> QKPKYQVRWKIIESYEGNSYTFIDPTQLPYNEKWEFPRNNLQFGKTLGAGAFGKVVEATAFGLGKEDAVLKVAVKMLKSTAHADEKEALMSELKIMSHLGQHENIVNLLGACTHGGPVLVITEYCCYGDLLNFLRRKAEAMLGPSLSPGQDPEGLDKEDGRPLELRDLLHFSSQVAQGMAFLASKNCIHRDVAARNVLLTNGHVAKIGDFGLARDIMNDSNYIVKGNARL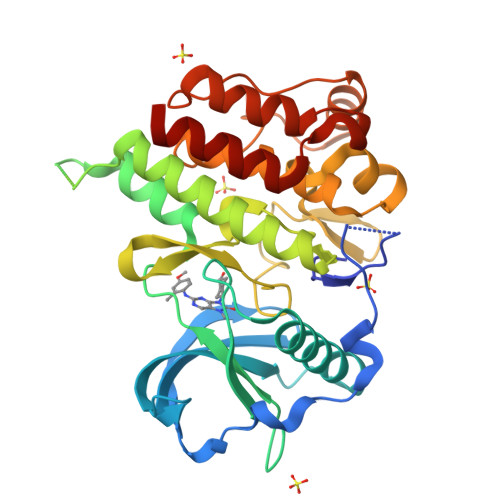PVKWMAPESIFDCVYTVQSDVWSYGILLWEIFSLGLNPYPGILVNSKFYKLVKDGYQMAQPAFAPKNIYSIMQACWALEPTHRPTFQQICSFLQEQAQEDRR The lectin pathway of complement is activated by complexes comprising a recognition component (mannose-binding lectin, serum ficolins, collectin-LK or collectin-K1) and a serine protease (MASP-1 or MASP-2). MASP-1 activates MASP-2, and MASP-2 cleaves C4 and C4b-bound C2. MASPs are homodimers that circulate as zymogens bound to the collagenous domains of MBL. Each MASP comprises two N-terminal CUB (C1r/C1s, Uegf, and bone morphogenetic protein-1) domains separated by an epidermal growth factor (EGF)-like domain followed by two short complement regulator (SCR) domains and a C-terminal serine protease (SP) domain.

In particular, MASP-2 CUB1-EGF-CUB2 (subsequently called MASP-2 3D) was crystallized in the presence of citrate that chelates Ca2+, and although Ca2+ was bound to the EGF-like domain, the CUB1 and CUB2 domains lacked Ca2+ and became partially disordered as a result (Feinberg et al., 2003). Because there was no structure of rat MASP-1 3D, and the existing structure of rat MASP-2 3D lacked two of the three Ca2+, including those Ca2+ that form part of the binding site for MBL, both rat MASP-1 3D and MASP-2 3D were crystallized in the presence of 2 mM calcium and diffraction data were collected. This resulted in one MASP-1 structure at 3.7 Å resolution and three independent MASP-2 structures at 2.6–2.7 Å resolution. For MASP-2 3D, 279 of 280 residues were visible. Interestingly, the three structures overlaid closely, with RMSDs of 0.682, 0.871, and 0.992 Å over 276 Cα atoms. The only notable differences were in the N-terminal seven residues and in a loop within the EGF-like domain (Thr125–Ser130), probably reflecting flexibility. A major difference, however, was that the structures now contained three bound Ca2+ compared with the single Ca2+ in the EGF-like domain of the earlier MASP-2 3D structure. In the MASP-2 CUB1 domain, Ca2+ formed contacts with six oxygen atoms in the side chains of Glu48, Asp56, Asp101, and Asn104 and the main chain oxygen of Ser103 (distances between 2.3 and 2.7 Å). In the MASP-2 CUB2 domain, Ca2+ formed contacts with five oxygen atoms at the side chains of Glu215, Asp225, Asp262, and Ser264. The firm identification in this study of the three Ca2+ sites in rat MASP-2 now resolves a key ambiguity of the earlier rat MASP-2 structure (Feinberg et al., 2003).

>SKWPEPVFGRLVSPGFPEKYGNHQDRSWTLTAPPGFRLRLYFTHFNLELSYRCEYDFVKLTSGTKVLATLCGQESTDTERAPGNDTFYSLGPSLKVTFHSDYSNEKPFTGFEAFYAAEDVDECRTSLGDSVPCDHYCHNYLGGYYCSCRVGYILHQNKHTCSALCSGQVFTGRSGFLSSPEYPQPYPKLSSCAYNIRLEEGFSITLDFVESFDVEMHPEAQCPYDSLKIQTDKREYGPFCGKTLPPRIETDSNKVTITFTTDESGNHTGWKIHYTSTA[2x]>[4x]MGNRGMEDLIPLVNRLQDAFSAIGQNADLDLPQIAVVGGQSAGKSSVLENFVGRDFLPRGSGIVTRRPLVLQLVNATTEYAEFLHCKGKKFTDFEEVRLEIEAETDRVTGTNKGISPVPINLRVYSPHVLNLTLVDLPGMTKVPVGDQPPDIEFQIRDMLMQFVTKENCLILAVSPANSDLANSDALKVAKEVDPQGQRTIGVITKLDLMDEGTDARDVLENKLLPLRRGYIGVVNRSQKDIDGKKDITAALAAERKFFLSHPSYRHLADRMGTPYLQKVLNQQLTNHIRDTLPGLRNKLQSQLLSIEKEVEEYKNFRPDDPARKTKALLQMVQQFAVDFEKRIEGSGDQIDTYELSGGARINRIFHERFPFELVKMEFDEKELRREISYAIKNIHGIRTGLFTPDMAFETIVKKQVKKIREPCLKCVDMVISELISTVRQCTKKLQQYPRLREEMERIVTTHIREREGRTKEQVMLLIDIELAYMNTNHEDFIGFANAQQRSNQMNKKKTSGNQDEILVIRKGWLTINNIGIMKGGSKEYWFVLTAENLSWYKDDEEKEKKYMLSVDNLKLRDVEKGFMSSKHIFALFNTEQRNVYKDYRQLELACETQEEVDSWKASFLRAGVYPERVGDKEKASETEENGSDSFMHSMDPQLERQVETIRNLVDSYMAIVNKTVRDLMPKTIMHLMINNTKEFIFSELLANLYSCGDQNTLMEESAEQAQRRDEMLRMYHALKEALSIIGNINTTTVSTPMPPPVDDSWLQVQSVPAGRRSPTSSPTPQRRAPAVPPARPGSRGPAPGPPPAGSALGGAPPVPSRPGASPDPFGPPPQVPSRPNRAPPGVPSRSGQASPSRPESPRPPFDL;>[8x]MGNRGMEDLIPLVNRLQDAFSAIGQNADLDLPQIAVVGGQSAGKSSVLENFVGRDFLPRGSGIVTRRPLVLQLVNATT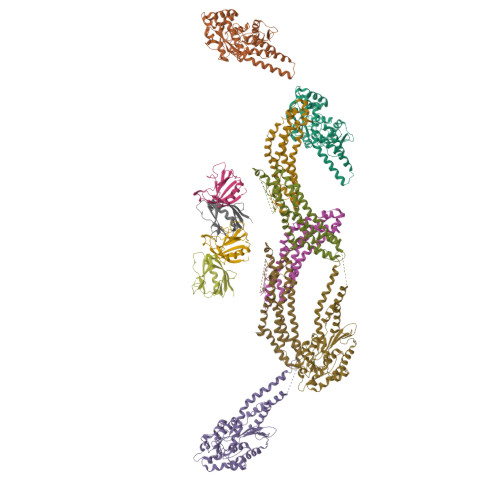EYAEFLHCKGKKFTDFEEVRLEIEAETDRVTGTNKGISPVPINLRVYSPHVLNLTLVDLPGMTKVPVGDQPPDIEFQIRDMLMQFVTKENCLILAVSPANSDLANSDALKVAKEVDPQGQRTIGVITKLDLMDEGTDARDVLENKLLPLRRGYIGVVNRSQKDIDGKKDITAALAAERKFFLSHPSYRHLADRMGTPYLQKVLNQQLTNHIRDTLPGLRNKLQSQLLSIEKEVEEYKNFRPDDPARKTKALLQMVQQFAVDFEKRIEGSGDQIDTYELSGGARINRIFHERFPFELVKMEFDEKELRREISYAIKNIHGIRTGLFTPDMAFETIVKKQVKKIREPCLKCVDMVISELISTVRQCTKKLQQYPRLREEMERIVTTHIREREGRTKEQVMLLIDIELAYMNTNHEDFIGFANAQQRSNQMNKKKTSGNQDEILVIRKGWLTINNIGIMKGGSKEYWFVLTAENLSWYKDDEEKEKKYMLSVDNLKLRDVEKGFMSSKHIFALFNTEQRNVYKDYRQLELACETQEEVDSWKASFLRAGVYPERVGDKEKASETEENGSDSFMHSMDPQLERQVETIRNLVDSYMAIVNKTVRDLMPKTIMHLMINNTKEFIFSELLANLYSCGDQNTLMEESAEQAQRRDEMLRMYHALKEALSIIGDINTTTVSTPMPPPVDDSWLQVQSVPAGRRSPTSSPTPQRRAPAVPPARPGSRGPAPGPPPAGSALGGAPPVPSRPGASPDPFGPPPQVPSRPNRAPPGVPSRSGQASPSRPESPRPPFDL> MGVFSKEQVQDMYALTPMQEGMLFHALLDQEHNSHLVQMSISLQGDLDVGLFTDSLHVLVERYDVFRTLFLYEKLKQPLQVVLKQRPIPIEFYDLSACDESEKQLRYTQYKRADQERTFHLAKDPLMRVALFQMSQHDYQVIWSFHHILMDGWCFSIIFDDLLAIYLSLQNKTALSLEPVQPYSRFINWLEKQNKQAALNYWSDYLEAYEQKTTLPKKEAAFAKAFQPTQYRFSLNRTLTKQLGTIASQNQVTLSTVIQTIWGVLLQKYNAAHDVLFGSVVSGRPTDIVGIDKMVGLFINTIPFRVQAKAGQTFSELLQAVHKRTLQSQPYEHVPLYDIQTQSVLKQELIDHLLVIENYPLVEALQKKALNQQIGFTITAVEMFEPTNYDLTVMVMPKEELAFRFDYNAALFDEQVVQKLAGHLQQIADCVANNSGVELCQIPLLTEAETSQLLAKRTETAADYPAATMHELFSRQAEKTPEQVAVVFADQHLTYRELDEKSNQLARFLRKKGIGTGSLVGTLLDRSLDMIVGILGVLKAGGAFVPIDPELPAERIAYMLTHSRVPLVVTQNHLRAKVTTPTETIDINTAVIG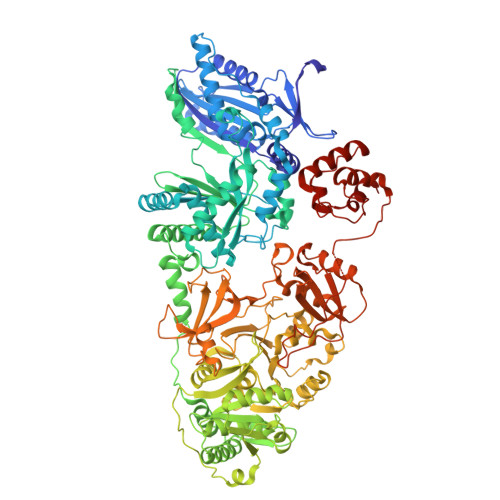EESRAPIESLNQPHDLFYIIYTSGTTGQPKGVMLEHRNMANLMHFTFDQTNIAFHEKVLQYTTCSFDVCYQEIFSTLLSGGQLYLITNELRRHVEKLFAFIQEKQISILSLPVSFLKFIFNEQDYAQSFPRCVKHIITAGEQLVVTHELQKYLRQHRVFLHNHYGPSETHVVTTCTMDPGQAIPELPPIGKPISNTGIYILDEGLQLKPEGIVGELYISGANVGRGYLHQPELTAEKFLDNPYQPGERMYRTGDLARWLPDGQLEFLGRIDHQVKIRGHRIELGEIESRLLNHPAIKEAVVIDRADETGGKFLCAYVVLQKALSDEEMRAYLAQALPEYMIPSFFVTLERIPVTPNGKTDRRALPKPEGSAKTKADYVAPTTELEQKLVAIWEQILGVSPIGIQDHFFTLGGHSLKAIQLISRIQKECQADVPLRVLFEQPTIQALAAYVELEHHHHHH>[2x]MAHHHHHHVDDDDKIQKTQSAPGTLSPDARNEKQPFYGEHQAGILTPQQAAMMLVAFDVLASDKADLERLFRLLTQRFAFLTQGGAAPETPNPRLPPLDSGILGGYIAPDNLTITLSVGHSLFDERFGLAPQMPKKLQKMTRFPNDSLDAALCHGDVLLQICANTQDTVIHALRDIIKHTPDLLSVRWKREGFISDHAARSKGKETPINLLGFKDGTANPDSQNDKLMQKVVWVTADQ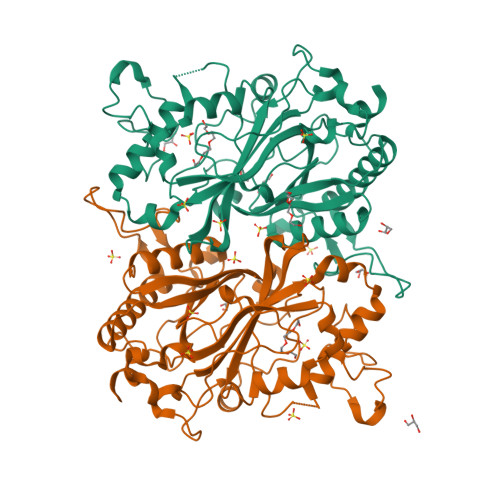QEPAWTIGGSYQAVRLIQFRVEFWDRTPLKEQQTIFGRDKQTGAPLGMQHEHDVPDYASDPEGKVIALDSHIRLANPRTAESESSLMLRRGYSYSLGVTNSGQLDMGLLFVCYQHDLEKGFLTVQKRLNGEALEEYVKPIGGGYFFALPGVKDANDYFGSALLRV>LSNEDPKDTLLREFQEEIARLKAQLEKKGMLVEDLEKERDFYFGKLRNIELICQENEGENDPV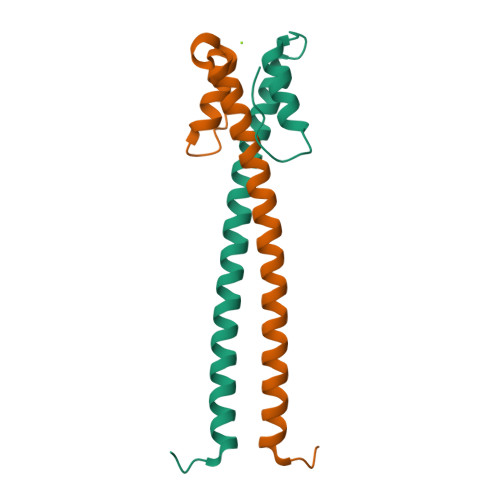LQRIVDILYATDEGFVIPD[2x]>TCPEQDKYRTITGMCNNRRSPTLGASNRAFVRWLPAEYEDGFSLPYGWTPGVKRNGFPVALARAVSNEIVRFPTDQLTPDQERSLMFMQWGQLLDHDLDFTPEPAARASFVTGVNCETSCVQQPPCFPLKIPPNDPRIKNQADCIPFFRSCPACPGSNITIRNQINALTSFVDASMVYGSEEPLARNLRNMSNQLGLLAVNQRFQDNGRALLPFDNLHDDPCLLTNRSARIPCFLAGDTRSSEMPELTSMHTLLLREHNRLATELKSLNPRWDGERLYQEARKIVGAMVQIITYRDYLPLVLGPTAMRKYLPTYRSYNDSVDPRIANVFTNAFRYGHTLIQPFMFRLDNRYQPMEPNPRVPLSRVFFASWRVVLEGGIDPILRGLMATPAKLNRQNQIAVDEIRERLFEQVMRIGLDLPALNMQRSRDHGLPGYNAWRRFCGLPQPETVGQLGTVLRNLKLARKLMEQYGTPNNIDIWMGGVSEPLKRKGRVGPLLACIIGTQFRKLRDGDRFWWENEGVFSMQQRQALAQISLPRIICDNTGITTVSK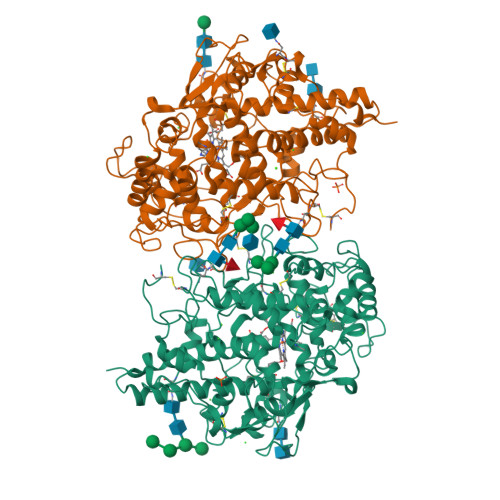NNIFMSNSYPRDFVNCSTLPALNLASWREA[8x]Ring-shaped enzymes called AAA+ unfoldases help to recycle these proteins by unfolding their amino acid chains. The 83 kDa VAT protein, which is composed of an N-terminal regulatory domain (NTD) and two tandem nucleotide-binding AAA+ domains (NBD1 and NBD2), assembles into a 500 kDa homohexamer. Truncation of the first 182 residues of VAT removes the regulatory NTD, producing a construct (ΔN-VAT) that has both higher ATPase and unfoldase activity than the intact protein. All AAA+ unfoldases have conserved sequences that extend from the NBDs towards the center of the ring, forming ‘pore loops’ that are essential for unfolding substrate.

Similarly, ΔN-VAT with bound ATPγS forms a mixture of fibrils as well as single particles, the majority of which appeared to be six-fold symmetric (red circles). Single particle cryo-EM analysis was performed, excluding the fibrils by inspecting micrographs after automatic particle selection and manually deselecting particle images that were part of a filament. This process allowed calculation of a cryo-EM map of the six-fold symmetric stacked-ring conformation of VAT at 3.9 Å resolution. First, removal of the NTDs in ΔN-VAT makes the complex more structurally homogeneous and allowed specimens to be prepared with thinner ice than could be used with full length VAT. In the structure, a central pore runs along the six-fold symmetry axis of the complex through the center of the stacked NBD1 and NBD2 rings (left, hexagon). In the six-fold symmetric VAT structure, pore loop 1 of NBD1, containing conserved and essential tyrosine residues (Tyr264 and Tyr265), forms an opening that is ~28 Å across while pore loop 2 of NBD1 (residues 299 to 305) forms a slightly tighter aperture that is ~18 Å across (left). Similar apertures are produced by the corresponding pore loop 1 of NBD2 (containing conserved residues Trp 541 and Val 542) and pore loop 2 of NBD2 (residues 575–579) (left). The stacked-ring structure of VAT resembles recent structures of the VAT homologue p97 in the fully ATP-loaded state, except for the orientations between the NBD1 and NBD2 domains in VAT protomers and the relative rotation of the NBD1 and NBD2 rings. Consequently, the six-fold symmetric stacked-ring state with ATPγS bound and the split-ring state with ADP bound likely correspond to pre- and post-unfolding conformations of the enzyme.

>MEVSRISYEDIGGLSEQLGKIREMIELPLKHPELFERLGITPPKGVILYGPPGTGKTLIARAVANESGANFLSINGPEIMSKYYGQSEQKLREIFSKAEETAPSIIFIDEIDSIAPKREEVQGEVERRVVAQLLTLMDGMKERGHVIVIGATNRIDAIDPALRRPGRFDREIEIGVPDRNGRKEILMIHTRNMPLGMSEEEKNKFLEEMADYTYGFVGADLAALVRESAMNALRRYLPEIDLDKPIPTEILEKMVVTEDDFKNALKSIEPSSLREVMVEVPNVHWDDIGGLEDVKREIKETVELPLLKPDVFKRLGIRPSKGFLLYGPPGVGKTLLAKAVATESNANFISIKGPEVLSKWVGESEKAIREIFKKAKQVAPAIVFLDEIDSIAPRRGTTSDSGVTERIVNQLLTSLDGIEVMNGVVVIGATNRPDIMDPALLRAGRFDKLIYIPPPDKEARLSILKVHTKNMPLAPDVDLNDIAQRTEGYVGADLENLCREAGMNAYRENPDATSVSQKNFLDALKTIRPSVDEEVIKFYRTLSETMSKSVSERRKQLQDQGLYL[6x]Here, we report the first crystal structure of an ecdysteroidogenic regulator encoded by the Halloween gene, noppera-bo (nobo). nobo encodes a member of the epsilon class of cytosolic GSH S-transferases (GST, EC 2.5.1.18; hereafter GSTEs). DmNobo forms a polypeptide homodimer with a canonical GST fold, which has a well-conserved GSH-binding site (G-site) and a hydrophobic substrate-binding pocket (H-site) adjacent to the G-site. Consistent with the requirement of GSH for GST function, a defect in GSH biosynthesis in D. melanogaster also leads to larval lethality, which is partly rescued by the administration of 20E or cholesterol. These data indicate that the nobo family of GSTs is essential for ecdysteroid biosynthesis by regulating cholesterol trafficking and/or metabolism. In general, GSTs catalyze various reactions with an activated glutathione (GSH) molecule in the following three ways: GSH conjugation to a substrate, reduction of a substrate using GSH, and isomerization.

The importance of the Asp-113–EST hydrogen bond for EST binding was biochemically examined with a recombinant mutated DmNobo protein carrying D113A amino acid substitution (DmNobo D113A). DmNobo D113A lacks the sidechain carboxyl group at position 113 and therefore cannot form a hydrogen bond with EST. The crystal structure of the DmNobo D113A did not show significant structural differences compared with the WT DmNobo (DmNobo WT) protein. In the absence of EST, both DmNobo WT and DmNobo D113A showed GSH conjugation activity although the activity of DmNobo D113A decreased by approximately half of DmNobo WT. In the presence of EST, as expected from the EST-binding to the H-site, the enzymatic activity of DmNobo WT was inhibited with an IC50 value of ∼2.3 μm. In contrast, the enzymatic activity of DmNobo D113A was not inhibited by EST, even at a concentration of 25 μm. In contrast, it was barely possible to determine the Kd value between DmNobo D113A and EST because of a weak interaction, which was consistent with crystal structure analysis.

>[2x]MNHKVHMMSQPKPILYYDERSPPVRSCLMLIKLLDIDVELRFVNLFKGEQFQKDFLALNPQHSVPTLVHGDLVLTDSHAILIHLAEKFDEGGSLWPQEHAERMKVLNLLLFECSFLFRRASDFMSAIVRQGFANVDVAHHERKLTEAYIIMERYLENSDFMAGPQLTLADLSIVTTLSTVNLMFPLSQFPRLRRWFTAMQQLDAYEANCSGLEKLRQTMESVGSFQFPSSSAVVTEKVE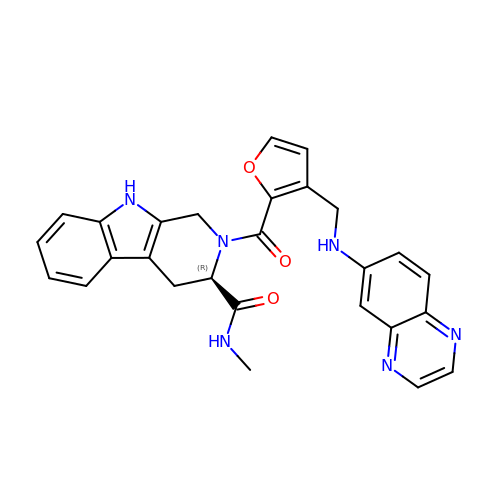(R)-N-methyl-2-(3-((quinoxalin-6-ylamino)methyl)furan-2-carbonyl)-2,3,4,9-tetrahydro-1H-pyrido[3,4-b]indole-3-carboxamide | C27 H24 N6 O3 | WHELPQVBBOUXAO-XMMPIXPASA-N>HHHHHHENLYFQSQCTVRYNVADCSHLKLTHIPDDLPSNITVLNLTHNQLRRLPPTNFTRYSQLAILDAGFNSISKLEPELCQILPLLKVLNLQHNELSQISDQTFVFCTNLTELDLMSNSIHKIKSNPFKNQKNLIKLDLSHNGLSSTKLGTGVQLENLQELLLAKNKILALRSEELEFLGNSSLRKLDLSSNPLKEFSPGCFQTIGKLFALLLNNAQLNPHLTEKLCWELSNTSIQNLSLANNQLLATSESTFSGLKWTNLTQLDLSYNNLHDVGNGSFSYLPSLRYLSLEYNNIQRLSPRSFYGLSNLRYLSLKRAFTKQSVSLASHPNIDDFSFQWLKYLEYLNMDDNNIPSTKSNTFTGLVSLKYLSLSKTFTSLQTLTNETFVSLAHSPLLTLNLTKNHISKIANGTFSWLGQLRILDLGLNEIEQKLSGQEWRGLRNIFEIYLSYNKYLQLSTSSFALVPSLQRLMLRRVALKNVDISPSPFRPLRNLTILDLSNNNIANINEDLL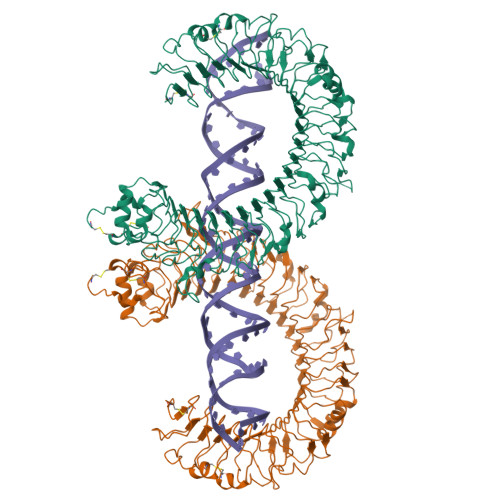EGLENLEILDFQHNNLARLWKRANPGGPVNFLKGLSHLHILNLESNGLDEIPVGVFKNLFELKSINLGLNNLNKLEPFIFDDQTSLRSLNLQKNLITSVEKDVFGPPFQNLNSLDMRFNPFDCTCESISWFVNWINQTHTNISELSTHYLCNTPHHYYGFPLKLFDTSSCK[2x]>MRCVGIGNRDFVEGLSGATWVDVVLEHGSCVTTMAKDKPTLDIELLKTEVTNPAVLRKLCIEAKISNTTTDSRCPTQGEATLVEEQDANFVCRRTFVDRGWGNGCGLFGKGSLLTCAKFKCVTKLEGKIVQYENLKYSVIVTVHTGDQHQVGNETTEHGTIATITPQAPTSEIQLTDYGALTLDCSPRTGLDFNEMVLLTMKEKSWLVHKQWFLDLPLPWTSGASTSQETWNRQDLLVTFKTAHAKKQEAVVLGSQEGAMHTALTGATEIQTSG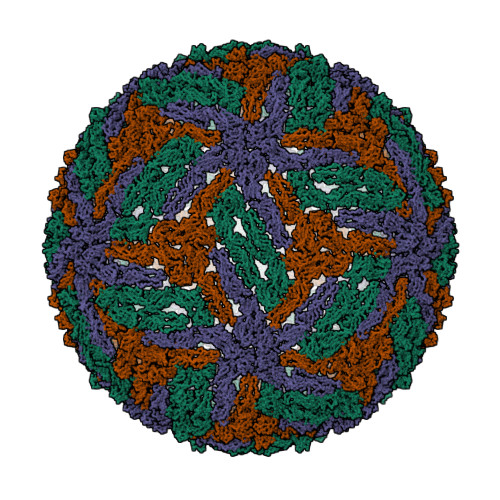TTTIFAGHLKCRLKMDKLTLKGISYVMCTGSFKLEKEVAETQHGTVLVQVKYEGTDAPCKIPFSSQDEKGVTQNGRLVTANPIVTDKEKPVNIEAEPPFGESYIVVGAGEKALKLSWFKKGSSIGK[3x]>ANSKLTSDFDNPRWIGRHKHMFNFLDVNHNGKISLDEMVYKASDIVINNLGATPEQAKRHKDAVEAFFGGAGMKYGVETDWPAYIEGWKKLATDELEKYAKNEPTLIRIWGDALFDIVDKDQNGAITLDEWKAYTKAAGIIQSSEDCEETFRVCDIDESG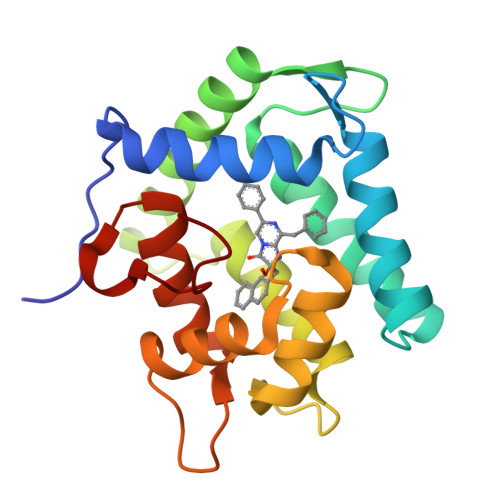QLDVDEMTRQHLGFWYTMDPACEKLYGGAVP[2x]> MKHTELRAAVLDALEKHDTGATFF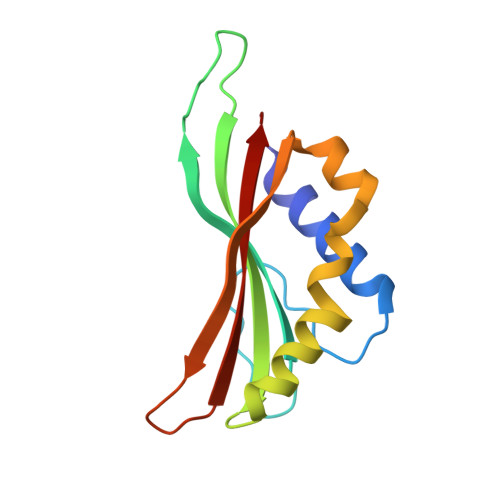DGRPAVFDEADFPAVAVYLTGAEYTGEELDSDTWQAELHIEVFLPAQVPDSELDAWMESRIYPVMSDIPALSDLITSMVASGYDYRRDDDAGLWSSADLTYVITYEM> MATSELSSEVSEENSERREAFWAEWKDLTLSTRPEEGSSLHEEDTQRHE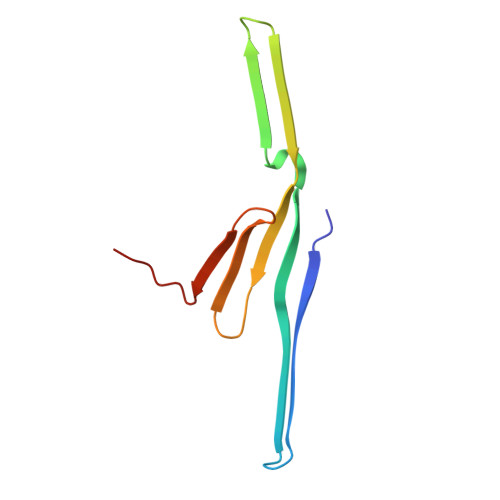TYHQQGQSQVLVQRSPWLMMRMGILGRGLQEYQLPYQRVLP1-cyclopropyl-2,5-dimethyl-pyrrole-3-carboxylic acid | C10 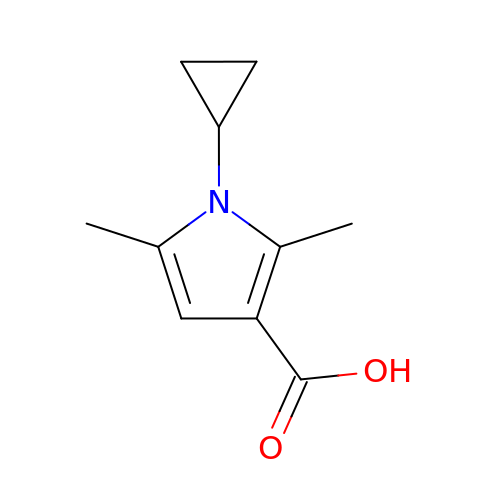H13 N O2 | VOOZJPFNBFNPEK-UHFFFAOYSA-N>MAHHHHHHMANGTQDGIQIRGSVPAIVTPMLEDGGLDLAAFRKLIDWHIEEGTDALVVVGTSGESATLSVDEHVLMIETAVKHAAKRIPIVA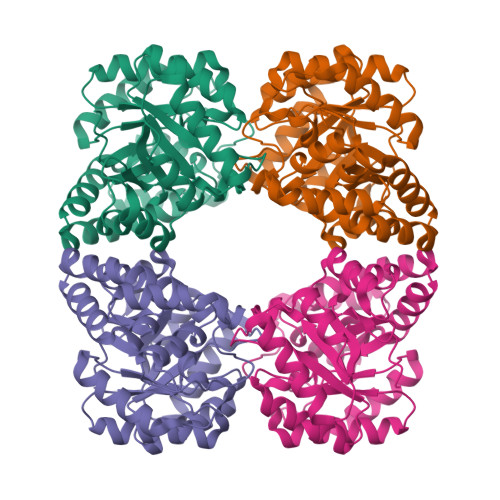GAGGNSTTEAIELSKHAKAVGADATLQVVPYYNKPTQEGIYRHFKAIAEAVDLPVILYNVPGRTVADMSNETTLRLAQVPGIIGVKDATGNIDRAAQLIKAAPAHFSIYSGDDPTAIALMLLGGHGNISVTANVAPRAMSELCRAALAADVKTAREIHMKLLSLHKHLFIEANPIPVKWALQQMGKIAGGIRLPLTPLDERCHETVRGALREAGLL[2x]>[6x]MDNQHKKIKGYRDLSQEEIDMMNRVKELGSQFEKLIQDVS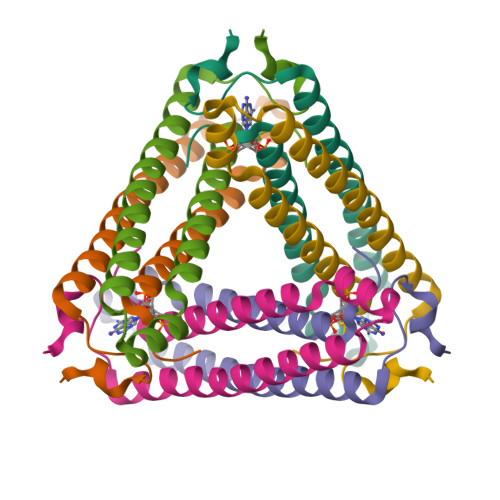DHLRGQYNASLHNRDEITRIANAEPGRWLAIGKTDIQTGMMAIIRAIAQPDSF>GSPPFTLPNLPVNNLSHSRVMEPIAQMMSSRNFPASVQFQNGRCTLSGDLLGTTPSSPSDLGAFVGLIAEPGSRVVELSQPNQEDFHAGSAPAPFGFPDFSDCSLTFVVASATTVGERTVNARSPQNFTPALGHITFDEEAPADLFRAHLRNLWDPTEHSFWRIPDYRADVLGSEFAPSVSAPGVGETLLFFMCNVPRLNGANPNPCPCLLPQEWITHFVSERAALQSDVALLNYVNPNTGRVLFEAKLYANGFLTVNLGASDQAT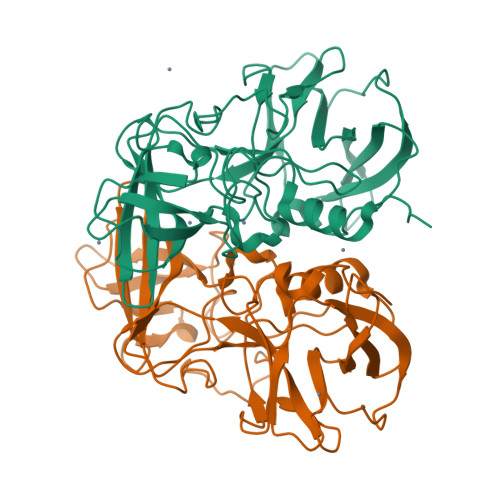LPVDGIFKFVSWVSFYYQLRPV[2x]>MWGKKDAGTELTNYQTLATNTIGMMKGVDGYAFTSGAKMTDTLIQAGAAKGMTVSGDPASGSATLWNSWGGQIVVAPDTAGGTGFNNGFTITTNKVPQSACVSISTGMSRSGGTSGIKINGNNHTDAKVTAEIASSECTADNGRTGTNTLVFNYNG[2x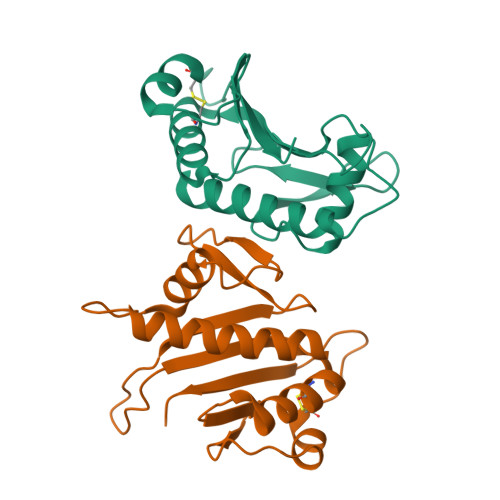]>MSLDAVGSLETKGFPGVLAAADAMVKTGRVTLVGYIRAGSARFTIIIRGDVSEVKTAMDAGIHAVDKAYGAALETWVIIPRPHENVECVLPIAYNENVERFRESTERPLIGSSQNRSWSHPQFEK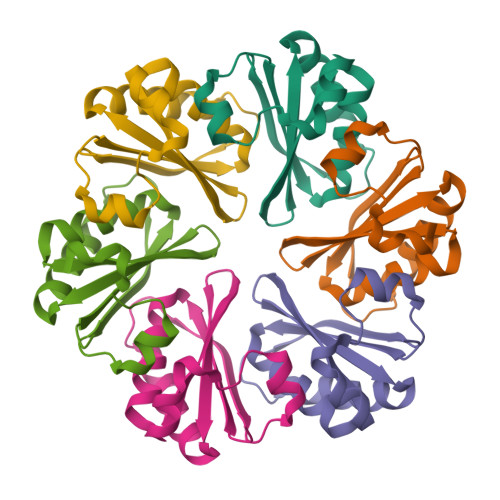[6x]> GPGSALRETVVEVPQVTWEDIGGLEDVKRELQELVQYPVEHPDKFLKFGMTPSKGVLFYGPPGCGKTLLAKAIANECQANFISIKGPELLTSEANVREIFDKARQAAPCVLFFDELDSIAKAADRVINQILTEMDGMSTKKNVFIIGATNRPDIIDPAILRPGRLDQLIYIPLPDEKSRVAILKANLRKSPVAKDVDLEFLAKMTNGFSGADLTEICQRACKLAIR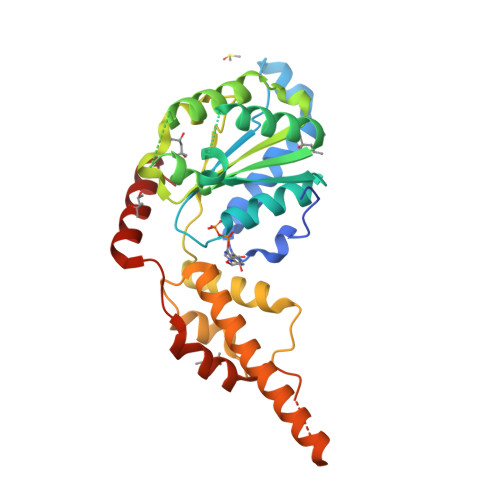ESIESEIRREREVPEIRRDHFEEAMRFARRSVSDNDIRKYEMFAQTLQQ> GPLGSATITQDTPINQIFTDTALAEKMKTVLGKTNVTDTVSQTDLDQVTTLQADRLGIKSIDGVEYLNNLTQINFSNNQLTDITPLKNLTKLVDILMNNNQIADITPLANLTNLTGLTLFNNQITDIDPLKNLTNLNRLELSSNTISDISALSGLTSLQQLSFGNQVTDLKPLANLTTLERLD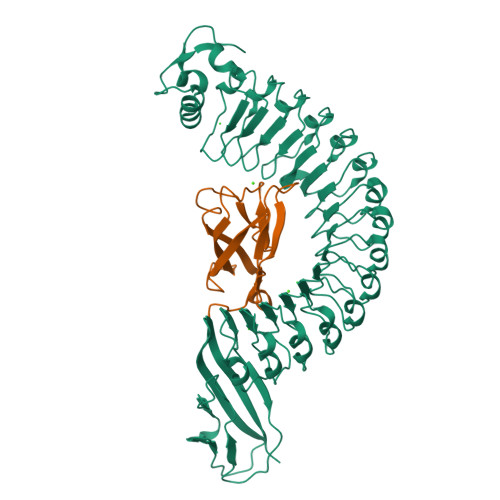ISSNKVSDISVLAKLTNLESLIATNNQISDITPLGILTNLDELSLNGNQLKDIGTLASLTNLTDLDLANNQISNLAPLSGLTKLTELKLGANQISNISPLAGLTALTNLELNENQLEDISPISNLKNLTYLTLYFNNISDISPVSSLTKLQRLFFYNNKVSDVSSLANLTNINWLSAGHNQISDLTPLANLTRITQLGLNDQAWTNAPVNYKANVSIPNTVKNVTGALIAPATISDGGSYTEPDITWNLPSYTNEVSYTFSQPVTIGKGTTTFSGTVTQPLKA;> GPLGSWVIPPISCPENEKGPFPKNLVQIKSNKDKEGKVFYSITGQGADTPPVGVFIIERETGWLKVTEPLDRERIATYTLFSHAVSSNGNAVEDPMEILITVTDQ> MEDDMACVKDLVSKYLADNERLSRQKLAFLVQTEPRMLLMEGLKLLSLCIEIDSCNANGCEHNSEDKSVERILHDHGILTPSLCFVVPDGYKLTGNVLILLECFVRSSPANFEQKYIEDFKKLEQLKEDLKSVDINLIPLIDGRTSFYNEQIPDWVNDKLRDTLFSLLRYAQESNSLFEESEYSRLCESLSMTSGRLSGVESLNVLLDNRSSHYEEIIASCHQGINNKLTAHEVKLQIEEEYQVFRNRLRKGEITGQFLKVDKSRLLNDFNNLYVDEVTATKDNIEHLIYQFKRASPILRFLYANIGEGNGEERHHTIKECQMQYWRSFLNKVKSLRILNTRRKLLLIFDALILLASIHDQTRHKCSKGWLGSCFISVNDRLVSLESTKRDLEKWVGRRQQSERSNTIQPPDKNQILISMFQKTILKATAALKDVGISVEHYKINMEVICPDSYDLILNFDVSGVVPTISYQRTEDEKFPFIMGGVELLESTDLERLSSLSLALVNSMKTSSTVKLRQNEFGPARYQVVRCKEAYCQEFLLSGAEFQLIYQKTGECSKCYAINDNRVGEICSFYADPKRYFPAIFSAEVLQTTVSTMISWVKDCSELEEQLCNINSLTKMILVLILAHPSKRSQKLLQNLRYFIMAYVSDYHHKDLIDKLREELITDVEFLLYRLVRALVNLILSEDVKSMMTNRFKFILNISYMCHFITKETPDRLTDQIKCFEKFLEPKLEFGHVSINPADVATEEELDDMVYNAKKFLSKEGCTSIKGPDYKKPGVSKRFLSLLTSSFNNGSLFKESEVKREIKDPLVTSGCATALDLASNKSVVVNKYTDGSRVLNYDFNKLTALAVSQLTEVFSRKGKHLLNKQDYDYKVQQAMSNLVLGPRQNKVGADEADLDEILLDGGASVYFDQLKETVERIIDQYREPVKPGSNPNGGDQPSVNDLDEVVPNKFYIRLIKGELSNHMVEDFDYDVLPGNFYEEFCDAVYKNNKLKERYFYCGQMSQCPIGELTKAVATRTYFDQEYFQCFKSILLIMNANTLMGRYTHYKSRNLNFKFDMGRLSDDVRISERESNSEALSKALSLTNCTTAMLKNLCFYSQESPQSYSSTGPDTGRLKFSLSYKEQVGGNRELYIGDLRTKMFTRLIEDYFEALSLQLSGSCLNNEREFENAILSMKLNVSLAHVSYSMDHSKWGPMMCPFLFLATLQNLIFLSKDLQADIKGRDYLSTLLTWHMHKMVEIPFNVVSAMMKSFIKAQLGLKKKTTQSITEDFFYSNFQIGVVPSHVSSILDMGQGILHNTSDFYALISERFINYAISCICGGTIDAYTSSDDQISLFDQVLTELMQRDPEEFKTLIEFHYYMSDQLNKFVSPKSVIGRFVAEFKSRFYVWGDEVPLLTKFVAAALHNIKCKEPHQLAETIDTIIDQSVANGVPVHLCNLIQKRTLSLLQYARYPIDPFLLNCETDVRDWVDGNRSYRIMRQIERLIPDACGRIRSMLRKLYNKLKTGQLHEEFTTNYLSSEHLSSLSNLCELLGVEPPSESDLEFSWLNLAAHHPLRMVLRQKIIYSGAVNLDDEKVPTIVKTIQNKLSSTFTRGAQKLLSEAINKSAFQSSIASGFVGLCRTLGSKCVRGPNKESLYIK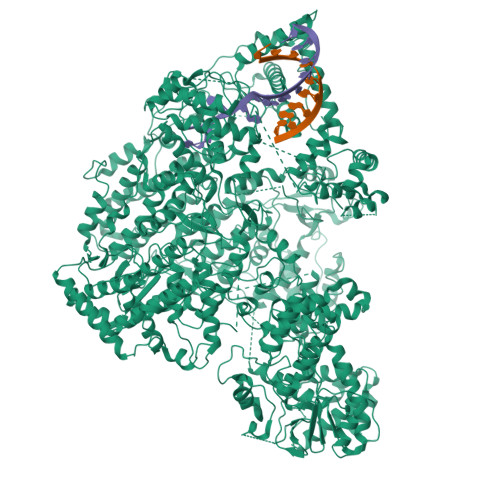SIQSLISDIQGIEPLIDSHGVQYWRVPLNIRDGNEGVISYFRPLLWDYMCISLSTAIELGAWVLGEPKKVRVLEFFKHNPCDYFPLKPAASKLLEDRVGLNHIIHSLRRLYPSVFEKHILPFMSDLASTKMKWSPRIKFLDLCVALDVNCEALSLVSHIVKWKREEHYIVLSSELRLSHTRTHEPMVEERVVSTSDAVDNFMRQIYFESYVRSFVATTRTLGSFTWFPHKTSVPEGEGLQRLGPFSSFVEKAIHKGIERPMFKHDLMMGYAWIDFDIEPARFNHNQLIASGLVGPRFDSLEDFFDAVESLPPGSAKLSQTVRFRIKSQDASFKESFAIHLDYTGSINQQTKYLVHEVSAMYSGAVSPCVLSDCWRLVLSGPTFKGKSAWYVDTEIVNEFLTDTNQLGHVTPVEIVVDMEKLQFTEYDFVLVGPCVEPVPLVVHRSGLWECDKKLASFTPVVQDQDLEMFVKEVGDSSLDLLIGALSAMILDRLKLRMQWSEVDIVSMLKAAMPSNSVKVLNAVLEAVDDWVDFKGYALCYSKSRKKVMVHSSGGKLRLKGRTCEELVKEDEGIEDIE> AMITEKSAALYARAVEVMPGGNSRTAVYSSPYPVYVRSGSGARVTDVDGVERIDFLNNSTTLIHGHAHPEMVEAIAAAVGHGTSFGMPTPVEVEYAEALSARNETFEHVRFTSSGTEAVMMAVQAARAYTERPKIAKIAGAYHGAYDAVAVNNDGSGNLISHAVTGNPEGVVANTVVIPFNDPEGSLEVLRRHADDLACVLIDPVPWRIGLLPASKEWLDALREFCDASGAVLISDEVGSYRVGYHGAMQLLGAEADITVMGKVIAAGMPIGAVAGRRRFMSVFDPSKGKPALPHSGSYNANPVSMSSGIASLRLLTPQAHERIGQLGEQARGSMRTALGEAGLDWEVNGLGSLFRVVANSAPAGYDSAAAAMKALYWKLLENG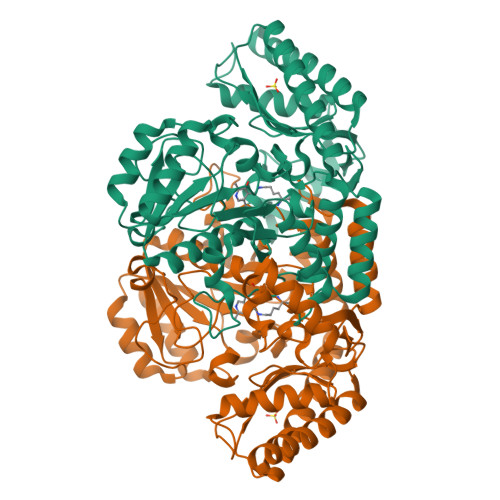IHIGDSGLGCISTPMGEEEIAEYAVAFAKSLGQVLAEGRA>[3x]SNAMATFMTEDFLLKNDIARTLYH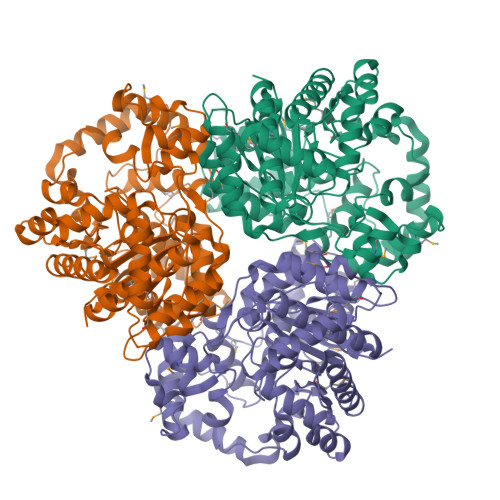KYAAPMPIYDFHCHLSPQEIADDRRFDNLGQIWLEGDHYKWRALRSAGVDESLITGKETSDYEKYMAWANTVPKTLGNPLYHWTHLELRRPFGITGTLFGPDTAESIWTQCNEKLATPAFSARGIMQQMNVRMVGTTDDPIDSLEYHRQIAADDSIDIEVAPSWRPDKVFKIELDGFVDYLRKLEAAADVSITRFDDLRQALTRRLDHFAACGCRASDHGIETLRFAPVPDDAQLDAILGKRLAGETLSELEIAQFTTAVLVWLGRQYAARGWVMQLHIGAIRNNNTRMFRLLGPDTGFDSIGDNNISWALSRLLDSMDVTNELPKTILYCLNPRDNEVLATMIGNFQGPGIAGKVQFGSGWWFNDQKDGMLRQLEQLSQMGLLSQFVGMLTDSRSFLSYTRHEYFRRILCNLLGQWAQDGEIPDDEAMLSRMVQDICFNNAQRYFTIK> GASKGNLLSPDRILTVAHRGASGYVPEHTILSYETAQKMKADFIELDLQMTKDGKLIVMHDEKLDRTTNGMGWVKDHTLADIKKLDAGSWFNEAYPEKAKPQYVGLKVPTLEEVLDRFGKHANYYIETKSPDTYPGMEEKLIASLQKHKLLGKHSKPGQVIIQSFSKESLVKVHQLQPNLPTVQLLEAKQMASMTDAALEEIKTYAVGAGPDYKALNQENVRMIRSHGLLLHPYTVNNEADMHRLLDWGVTGVFTNYPDLF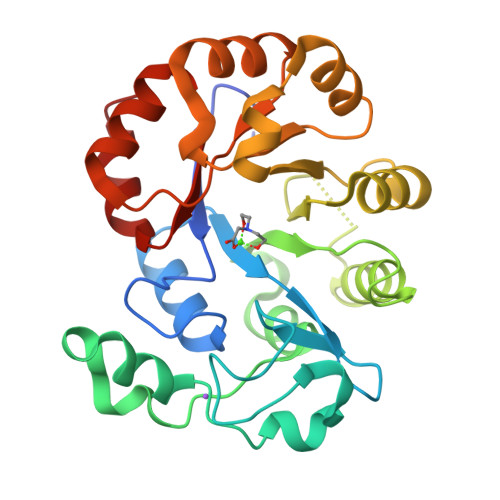HKVKKGY> MR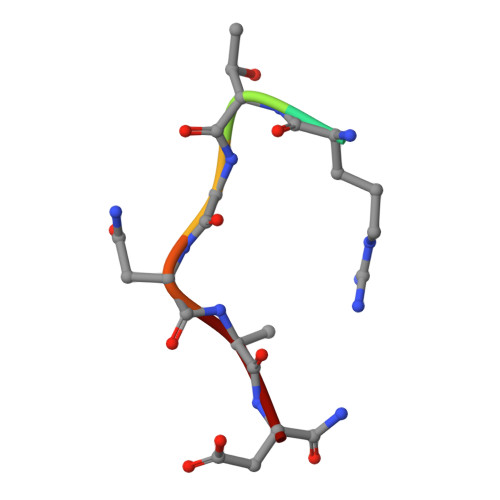TGNAN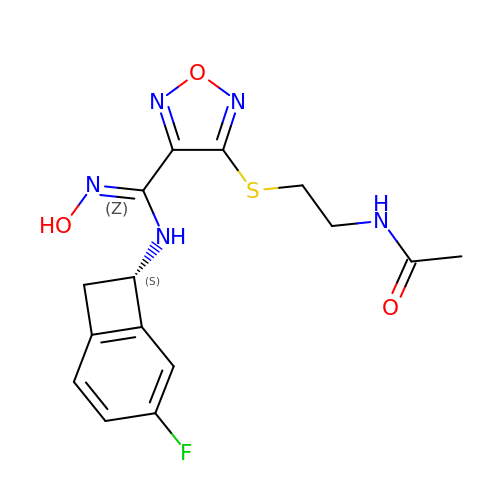N-{2-[(4-{N-[(7S)-4-fluorobicyclo[4.2.0]octa-1,3,5-trien-7-yl]-N'-hydroxycarbamimidoyl}-1,2,5-oxadiazol-3-yl)sulfanyl]ethyl}acetamide | C15 H16 F N5 O3 S | IWTLWDCOKRYTFP-LBPRGKRZSA-N>[2x]MGILKTLSAPIILENSNSTFTFLPGGDNFEWIHESIMINAFQGNTLDGSTNNLYLRIYKDNSLAFYPLIGMNSKSTIKSGTSTLIFEGTAEDISYTVTFRLTPYGIWFWDISLSGNCNKADIIYSQDIGVGTKGSVNSNELYLAQYLGHSIFQGDYGYVICSRQNMAQGDLFPYLQQGSLGIRSIAYSTDGTQFFGLSYKKTNIPEALYGDLPSKNKQYELAHTALQTEAFSLSGTKQFSFYGICKTNHPEVIREIEYIQELEKAYAYHESGEILPVNVPTLQNIGAPYASSRWDAKQVEHYFPKRLLEEKEEEALLSFFTPEKSHVVLQDKELTTERPHGHILMTNFDVTKVPQGVVSSTNYMYGAFNCQFVVGNTTYNKLLSNHRGLLNIQKDSGQRIFIKIGDCYRQLTLPAAYEMNVAGSTWYYQLDEDVLIITSFAMYNRPEIVLKVQSLGHKKYDFIVTHQLTVGPNEYENEIKLTREGNILQLSPTDPVVTNHFYPELSFRMRIPEDCTLSDDSIFFHNNTTINPSLLSIEILQKSSFDIVMQGFDTGNVIPFLDQYDYKEQLEAYRIYYDQLVCNFKLSAPDKIPLSAEKLNAIIHWYAHDALIHFASPHGLEQSGGAAWGTRDVCQGPIEFFLTTGHFDLVRHILITLYSHQIEGGFEWPQWFMFDHYPIHQEDCHGDVVFWPLKAISDYIQATGDTSILNELVDYRTAKDALPTNQPETILIHIKRAVTTIKNRYLSGTALISYAGGDWDDTLQPANSELKENLVSAWTQALAEQTLELLCSAIKGIDHDFSKELSHMANDIRTSFYQYLIKDGVIAGFLYRESEEHMKYMLHPDDTESSIHYRLLPLTRSIIAQLADFKLATRNLEIIDEHLACPDGVRLMDHPASYSGGISKIFLRAEQAANVGREISLQYVHAHIRYIEALATMGLSKKAWDALMRINPILLTDYVPNALTRQSNVYFSSSEGCFDDRYEYAKNFDKLRTGDINVKGGWRLYSSGPGIYIRRIIADLLGIRFGHNVIHIDPVVTKELDGVTLQFTCFGKTVFFTYHVDDTMDKHICVKSNNNILPGDNLNNIYRDGGIQIAKDVFLSAAMSDNNFHIYVKNLEHHHHHH

In this study, we identified the function of LpSOGP, determined its crystal structure, which is the first one among phosphorylases acting on β-linked glucan, and clarified the binding modes of substrates. In addition, LpSOGP did not show phosphorolytic activity toward cellobiose or laminaribiose. These results indicate that LpSOGP is highly specific to SopNs, as LiSOGP is, and is completely different from other GH94 enzymes in substrate specificity. The tertiary structure consists of four domains: two N-terminal β-sandwich domains (residues 1–257, yellow, Ndom1; and 295–553, light blue, Ndom2), a catalytic (α/α)6 barrel domain (593–1020, green), and a β sheet domain (magenta). Ndom1 is unique to LpSOGP, being missing in CBP, ChBP, and CBAP.

The crystal structure of apo LpSOGP was determined at 2.0 Å resolution. The crystals contain two identical molecules in an asymmetric unit. The two molecules in the asymmetric unit are in contact with each other mostly in the Ndom1 region. The contact area is only 2.5% (935.5 Å2) of the monomer surface area. The overall structure of LpSOGP besides Ndom1 is basically similar to those of GH94 CBAP from Saccharophagus degradans (SdCBAP), ChBP from Vibrio proteolyticus (VpChBP), and CBP from Cellvibrio gilvus (CgCBP) (the RMSD values are 4.11, 3.53, and 3.29 Å, respectively). As for the substrate recognition region, two helices (α1 and α2) in Ndom1 constitute a part of the catalytic pocket as well as in Ndoms in VpChBP and CgCBP. Ndom1 appears to be generated through domain duplication according to its position and the structural similarity to Ndom2. This duplication monomerizes LpSOGP but retains the fundamental constitution of a catalytic pocket between hetero domains.>MVQTGHRSLTSCIDPSMGLNEEQKEFQKVAFDFAAREMAPNMAEWDQKELFPVDVMRKAAQLGFGGVYIQTDVGGSGLSRLDTSVIFEALATGCTSTTAYISIHNMCAWMIDSFGNEEQRHKFCPPLCTMEKFASYCLTEPGSGSDAASLLTSAKKQGDHYILNGSKAFISGAGESD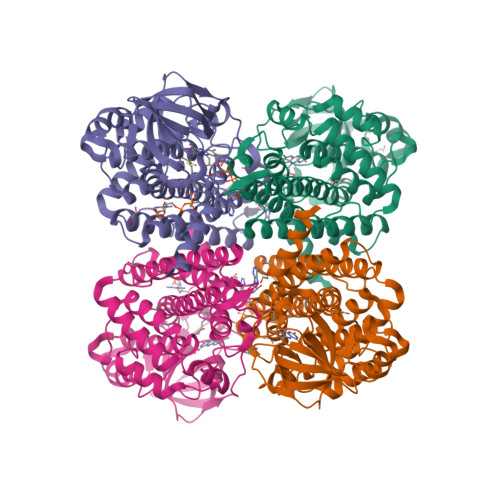IYVVMCRTGGPGPKGISCIVVEKGTPGLSFGKKEKKVGWNSQPTRAVIFEDCAVPVANRIGSEGQGFLIAVRGLNGGRINIASCSLGAAHASVILTRDHLNVRKQFGEPLASNQYLQFTLADMATRLVAARLMVRNAAVALQEERKDAVALCSMAKLFATDECFAICNQALQMHGGYGYLKDYAVQQYVRDSRVHQILEGSNEVMRILISRSLLQE[4x]>[2x]VLDGPYQPASFDLPVGNWMLLAPTGPGVVVEGTDNSGRWLSVILIEPGVTSETRTYTMFGSSKQVLVSNASDTKWKFVEMMKTAIDGDYAEWGTLLSDTK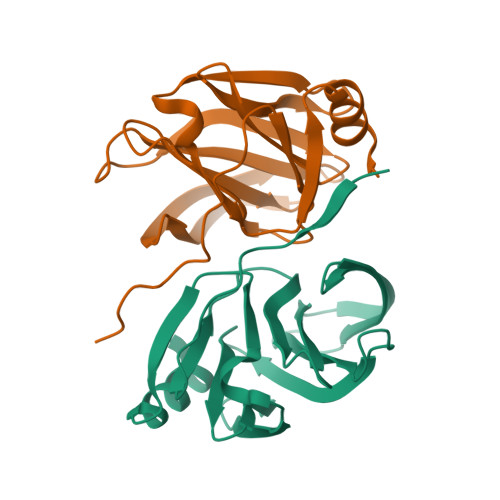LYGMMKYRKRLFIYEGETPNATTKRYIVTNYASVEVRPYSDFYIISRSQESACTEYINNGL>SNAQVEVIVMMHGRSTATSMVETVQ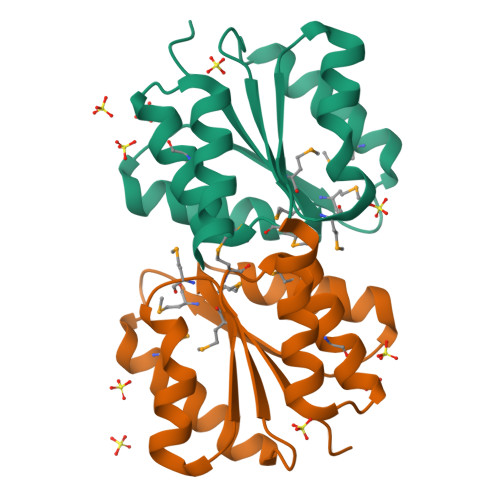ELLSIESGIALDMPLTVEVKAMYEKLKQTVVKLNPVKGVLILSDMGSLTSFGNILTEELGIRTKTVTMVSTPVVLEAMRKASLGRGLEDIYQSCEQLFENKYKAH[2x]Riboswitches are structured RNA elements that regulate gene expression upon binding to small molecule ligands. One class of commonly identified riboswitches are responsible for sensing the PreQ1 metabolite (7-aminomethyl-7-deazaguanine). Class I riboswitches feature a singular aptamer domain that directly interacts with PreQ1, initiating transcriptional attenuation or termination and in some cases inhibition of translational initiation. Multiple X-ray co-crystal structures of synthetic ligands with the Thermoanaerobacter tengcongensis (Tte)-PreQ1 riboswitch confirm a common binding site with the cognate ligand, despite considerable chemical differences among the ligands.

The co-crystal structures of the abasic mutant at positions 13, 14, and 15 in Tte-PreQ1 riboswitch aptamer (ab13_14_15) with 4 and 8 were determined at 2.15 A and 2.25 A resolution, respectively, by molecular replacement method. Compound 4 binds at the PreQ1 binding site, where the xanthone core is sandwiched by one face with G11 and the other with G5 and C16, residues that are strictly conserved in the class I PreQ1 riboswitches. However, because 4 is bulkier than PreQ1 and its heteroatom content is less than that of PreQ1, the binding pose of 4 slightly diverges from that of PreQ1. In contrast, the corresponding side of the xanthone moiety of 4 is further from these crucial atoms, resulting in a tilted binding axis of the heterocyclic core of 4 compared to PreQ1 of approximately 15 degrees. Consequently, the oxygen atom of the central ring of 4 is situated at 3.6 A away from the N6 atom of the phylogenetically conserved A29. This finding suggests a weak hydrogen bonding interaction between the riboswitch and compound 4, unlike the strong interaction observed in the PreQ1-bound form where the distance between the N6 atom of A29 and the N3 atom of PreQ1, a counterpart of the oxygen atom of the central pyranoid ring of 4, is 3.1 A . Superimposition of these two structures indicates that 4 collides with the base of C15 of the PreQ1-bound structure, due to the size of 4 being larger than that of PreQ1. Consequently, the conformation of the sugar and phosphate backbone at position 15 of the current structure is relocated to fit 4 into the ligand binding site, when compared to the PreQ1-bound form. Therefore, the binding of 4 to the PreQ1 binding site would affect the conformations of L2 and S3 that are important for regulating the riboswitch function. Consistent with this, the co-crystal structure with 4 exhibits conformational differences of L2 and S3 when compared to those in the PreQ1-bound form.

> CUGGGUCGCAGUNNNCCCAGUUAACAAAACAAG>MDTQHSALNARKQQATPRGVGVMCQWYAEKAENATIWDKEGNQFIDFAGGIAVLNTGHRHPKVIAAVTEQLTKFTHTAYQVTPYESYVALAERINERAPIAGPAKAAFFTTGAEAVENAVKIARCYTGRHGIITFGNGFHGRSFMTMAMTGKTAPYKRDFGVMPAGVFHARYPVPAKGISVDAAIESVEDIFSEDIAPHDVAAIVLEPVQGEGGFNVVPAEFLKRLRAICDKHGILLVADEVQSGFARTGKLFAMNHYETKADLITMAKSLGGGFPISGVVGRAEVMDAPNPGGLGGTYAGSPIAVAAAHAVIDAIEEENLCDRANELGAELVATLKDIQQATGDVVTDIRALGSMV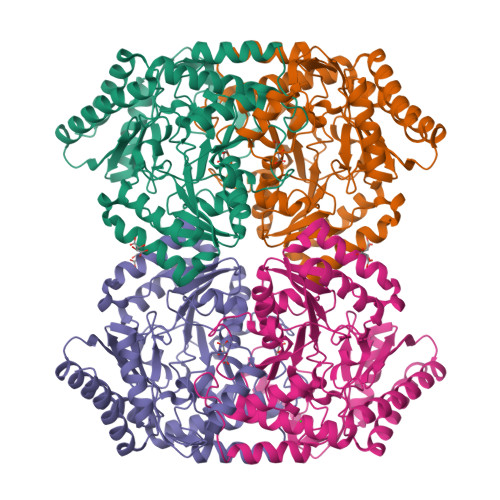AVELETAEQAKVVQNYAMENGLLLLTCGKYGNVIRFLYPLTIPAEQFRQGLDILKQGFATLKAGSAKAMEQSA[2x]> MIEDEMSREQIIKDGGNILVTAGAGSGKTTILVSKIEADLKENKTHYSIAAVTFTNKAAKEIEGRLGYSSRGNFIGTNDGFVESEIIRPFIKDAFGNDYPDNFTAEYFDNQFASYDKGLQVLKYQNILGTYSNPKKNFKFQLALDILKKSLVARQYIFSKYFKIFIDEYQDSDKDMHNLFMYLKDQLKIKLFIVGDPKQSIYIWRGAEPENFNGLIENSTDFNKYHLTSNFRCCQDIQNYSNLFNEETRSLIKEKNEVQNVISIADDMPISDILLKLTEEKQVLNIEAELVILVRRRNQAIEIMKELNEEGFNFIFIPQTPLDRATPNATLLKEVIKYVKNDRYSIYDLAAEIVGNLSSREIKEIQKIINELLVPNINQVLINQVLINLFAKLEITLDTREITAFTEVMMTNEFDIAFDTNEYLHKIFTVHSAKG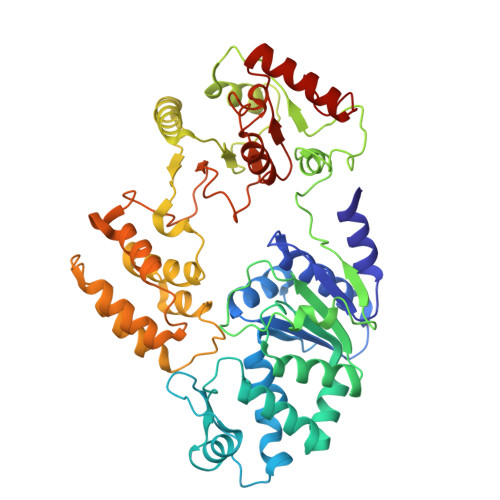LEFNQVIITASDYNVHYNRDTNEHYVATTRAKDKLIVIMDNKKYSDYIETLMKELKIKNIIKSI>[2x]GSLNITENESISTAVIDAINSGATLKDINAIPD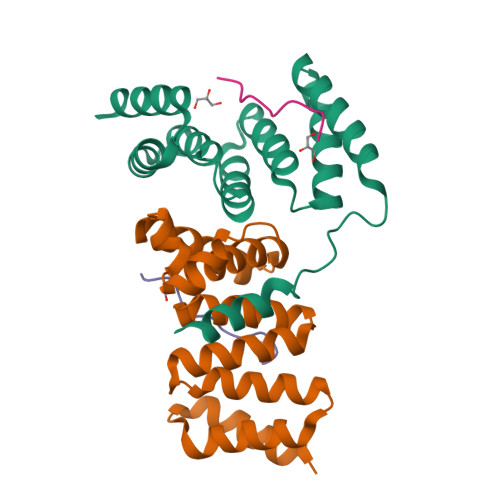DMMDDIYSYAYDFYNKGRIEEAEVFFRFLCIYDFYNVDYIMGLAAIYQIKEQFQQAADLYAVAFALGKNDYTPVFHTGQCQLRLKAPLKAKECFELVIQHSNDEKLKIKAQSYLDAIQ;>INTTNAHSTSNILIPELKAPKS[2x]>[6x]HPETLVKVKDAEDQLGARVGYIELDLNSGKILESFRPEERFPMMSTFKVLLCGAVLSRVDAGQEQLGRRIHYSQNDLVEYSPVTEKHLTDGMTVRELCSAAITMSDNTAANLLLTTIGGPKELTAFLHNM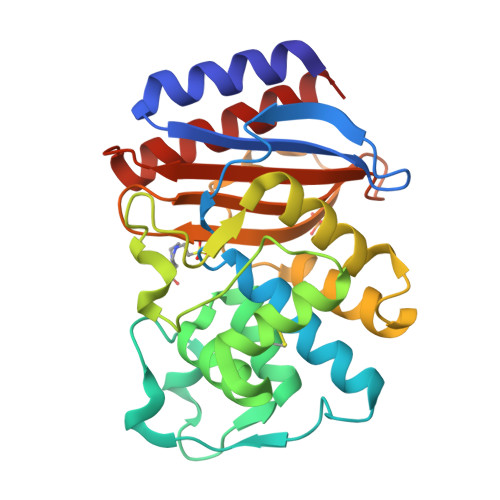GDHVTRLDRWEPELGEAIPNDERDTTMPAAMATTLRKLLTGELLTLASRQQLIDWMEADKVAGPLLRSALPAGWFIADKSGAGERGSRGIIAALGPDGKPSRIVVIYTTGSQATMDERNRQIAEIGASLIKHW>MNQNLLVTKRDGSTERINLDKIHRVLDWAAEGLHNVSISQVELRSHIQFYDGIKTSDIHETIIKAAADLISRDAPDYQYLAARLAIFHLRKKAYGQFEPPALYDHVVKMVEMGKYDNHLLEDYTEEEFKQMDTFIDHDRDMTFSYAAVKQLEGKYLVQNRVTGEIYESAQFLYILVAACLFSNYPRETRLQYVKRFYDAVSTFKISLPTPIMSGVRTPTRQFSSCVLIECGDSL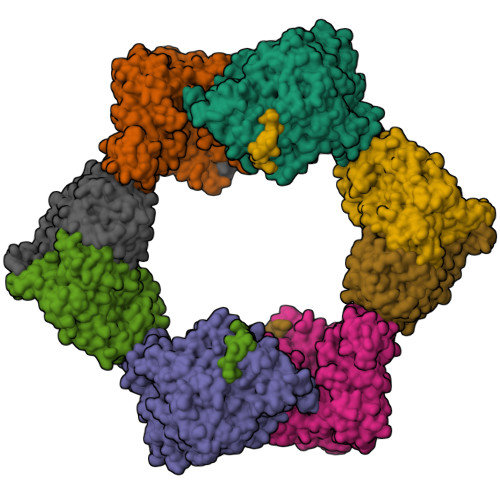DSINATSSAIVKYVSQRAGIGINAGRIRALGSPIRGGEAFHTGCIPFYKHFQTAVKSCSQGGVRGGAATLFYPMWHLEVESLLVLKNNRGVEGNRVRHMDYGVQINKLMYTRLLKGEDITLFSPSDVPGLYDAFFADQEEFERLYTKYEKDDSIRKQRVKAVELFSLMMQERASTGRIYIQNVDHCNTHSPFDPAIAPVRQSNLCLEIALPTKPLNDVNDENGEIALCTLSAFNLGAINNLDELEELAILAVRALDALLDYQDYPIPAAKRGAMGRRTLGIGVINFAYYLAKHGKRYSDGSANNLTHKTFEAIQYYLLKASNELAKEQGACPWFNETTYAKGILPIDTYKKDLDTIANEPLHYDWEALRESIKTHGLRNSTLSALMPSETSSQISNATNGIEPPRGYVSIKASKDGILRQVVPDYEHLHDAYELLWEMPGNDGYLQLVGIMQKFIDQSISANTNYDPSRFPSGKVPMQQLLKDLLTAYKFGVKTLYYQNTRDGAEDAQDDLVPSIQDDGCESGACKI[4x];>AYTTFSQTKNDQLKEPMFFGQPVNVARYDQQKYDIFEKLIEKQLSFFWRPEEVDVSRDRIDYQALPEHEKHIFISNLKYQTLLDSIQGRSPNVALLPLISIPELETWVETWAFSETIHSRSYTHIIRNIVNDPSVVFDDIVTNEQIQKRAEGISSYYDELIEMTSYWHLLGEGTHTVNGKTVTVSLRELKKKLYLCLMSVNALEAIRFYVSFACSFAFAERELMEGNAKIIRLIARDEALHLTGTQHMLNLLRSGADDPEMAEIAEECKQECYDLFVQAAQQEKDWADYLFRDGSMIGLNKDILCQYVEYITNIRMQAVGLDLPFQTRSNPIPWINTWLVSDNVQVAPQEVEVSSYLVGQIDSEVDTDDLSNFQL[4x]TRAF-interacting protein with a forkhead-associated (FHA) domain (TIFA) was originally identified as an adaptor protein that interacts with TRAF2 and TRAF61–3. TIFA has an FHA domain, involved in its binding to phosphothreonine (pThr), and has a consensus TRAF6-binding motif [PXEXX(Ar/Ac); Ar, aromatic; Ac, acidic; X, any] at the C-terminus for interaction with the TRAF-C domain of TRAF6 (TRAF6-C). Furthermore, oligomeric forms of TIFA promote oligomerisation and polyubiquitination of TRAF6, leading to the activation of IκB kinase (IKK). TIFA exists as an intrinsic dimer, and phosphorylation of TIFA at Thr9 promotes its oligomerisation through the intermolecular interaction of pThr9 with the FHA domain between the dimers.

Size-exclusion chromatography experiments of T9D/C36S and T9E/C36S showed that the phosphorylation-mimicking at Thr9 is partially involved in the TIFA assembly in solution (discussed later). Although it is difficult to discuss the original effect of pThr9 on oligomerisation even with the use of these results, the crystal structures of T9D/C36S and T9E/C36S provided structural insights into the assembly of TIFA. The TIFA hexamer in the T9D/C36S crystal shows a large buried surface area of approximately 1,400 Å2 per dimer, and the interactions between the dimers are also observed in the crystal of T9E/C36S.

>MSTFEDADEEETVTCLQMTIYHPGQQSGIFKSIRFSSKEKFPSIEVVKFGRNSNMCQYTFQDKQVSRIQFVLQPFKQFNSSVLSFEIKNMSKKTSLMVDNQELGYLNKMDLPYKCMLRFGEYQFLLQKEDGESVESFETQFIMSSRPLLQENNWPTQNPIPEDGMYSSYFTHRSSPSEMDENELLEHHHHHH[6x]> MGSSHHHHHHSQDPNSMKRLKDLREYLAVLEAHQDVREIDEPVDPHLEAGAAARWTYENRGPALMLNDLTGTGRFCRILAAPAGLSTIPGSPLARVALSLGLDVSATAHEIVDSLAAARTREPVAPVVVDSAPCQDNVLLGDDANLDRFPAPLLHEGDGGPYLNTWGTIIVSTPDGSFTNWAIARVMKIDGKRMTGTFIPTQHLGQIRKLWDNLGQPMPFAIVQGTEPGIPFVASMPLPDGIEEVGFLGAYFGEPLELVRAKTVDLLVPASAEIVI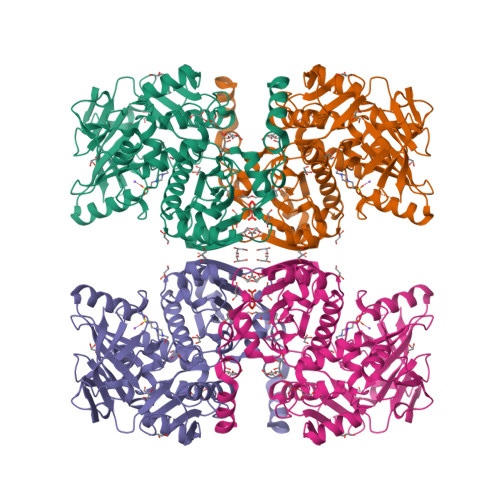EGHVMPGRTAVEGPMGEYAGYQPRHTSMQPEYVVDAITYRDDPIWPISVAGEPVDETHTAWGLVTAAEALALLRAAKLPVATAWMPFEAAAHWLIVCLTEDWRERMPGLSRDGICLRISQVLAATRIEAMMTRVFVLDDDVDPSDQTELAWAIATRVSPAHGRLVRHGMINPLAGCYSAEERRLGYGPKAVLNGLLPPMAERSRRSSFRHTYPEPVRQRVIELLA>[2x]HMLEMIKSGKARAHTNIALIKYWGKKDEALIIPMNNSISVTLEKFYTETKVTFNDQLTQDQFWLNGEKVSGKELEK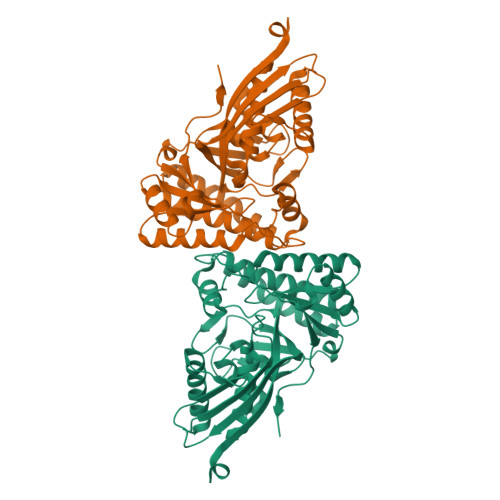ISKYMDIVRNRAGIDWYAEIESDNFVPTAAGLASSASAYAALAAACNQALDMQLSDKDLSRLARIGSGSASRSIYGGFAEWEKGYSDETSYAVPLESNHFEDDLAMIFVVINQHSKKVPSRYGMSLTRNTSRFYQYWLDHIDEDLAEAKAAIQDKDFKRLGEVIEENGLRMHATNLGSTPPFTYLVQESYDVMALVHECREAGYPCYFTMDAGPNVKILVEKKNKQQIIDKLLTQFDNNQIIDSDIIATGIEIIE> SNAMEILYIKGDATAPIGSGVKVITHICNDIGGWGKGFVLALSKKWKMPEEAYRQWYKSQEEFTLGAVQFVNVENKLYVANM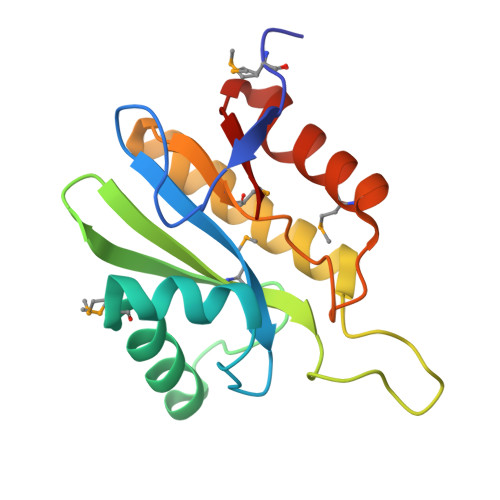IGQHGIYKDSKGLPPIRYDAVRQCLKEVALFTIAHKASVHMPRIGCGLAGGKWELMEQIIKEELITKEIAVTVYDL> MNEADYLRLLTRQAEQANDFLSNARKWDRERWVCQRFLEALNVPYRQEDFAAPGEQPPDVLFKGAGFEVFFVLDEGRRLNEEWREELTRRRQAVSLRQLIRREERPQRIAAAELQARLAPTLRKKAHNYSERGIDHGELDLLAFVNLKRAVPDFNTPFPPPTEYLRQGWRSLSMVGPT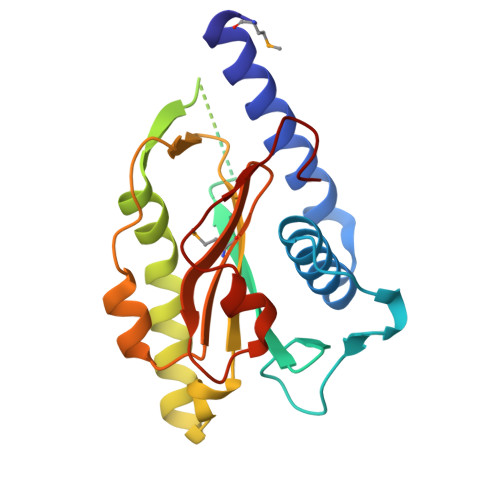FARVLFAHSGAPEFLRANLGRSILFDAGVGL> RRHVLLQAEFYQRSEGPDKAWAQFGFHFDADELFHVELDAAQTVWRLPEFGRFASFEAQGALQNMAVGKQNLEVMISNSNRSQQDFVTPELALFPAEAVSLEEPNVLICYADKFWPPVATMEWRRNGAVVSEGVYDSVYYGRPDLLFRKFSYLPFVPQRGDVYSCAVRHWGAEGPVQRMWEPE;> PANKMSMSTMNMPMAMKVGGGGSGGGGSGGGGSSAFFFCGAISECHYLNGTERVRYLQRYIYNRQQYAHFDSDVGKFVADSPLGEPQAEYWNSNAELLENRMNEVDRFCRHNYGGVESFTVQRSVEPKVRVSALQSGSLPETDRLACYVTGFYPPEIEVKWFLNGREETERV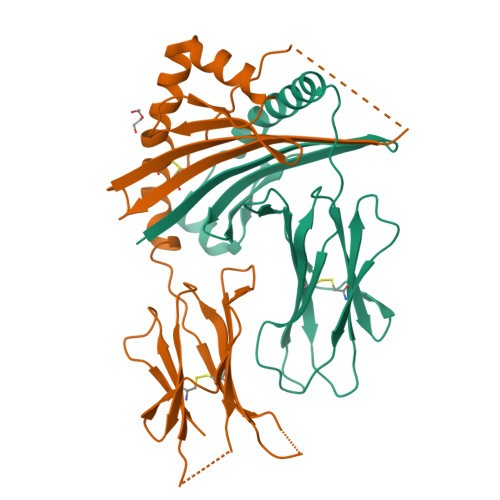VSTDVMQNGDWTYQVLVVLETVPRRGDSYVCRVEHASLRQPISQAWE> SRLIFEHQRRLTPPTTRKGTITIEPPPQLPRVVPPSLLRRVLPFLIVILIVGMIVALFATGMRLISPTMLFFPFVLLLAA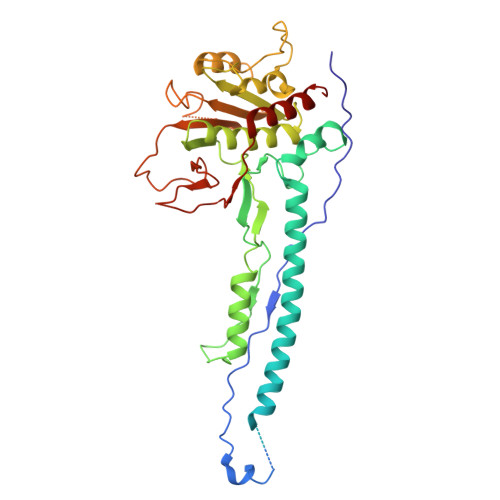TALYRGGDNKMRTEEVDAERADYLRYLSVVRDNVRAHAAEQRAALEWSHPEPEVLATIPGTRRQWERDPRDRDFLVLRAGRHDVPLDAALKVKDTADEIDLEPVAHSALRGLLDVQRTVRDAPTGLDVAKLARITVIGEADEARAAIRAWIAQAVTWHDPTMLGVALAAPDLESGDWSWLKWLPHVDVPNEADGVGPARYLTTSTAELRERLAPALADRPLFPAESGAALKHLLVVLDDPDADPDDIARKPGLTGVTVIHRTTELPNREQYPDPERPILRVADGRIERWQVGGWQPCVDVADAMSAAEAAHIARRLSRWDS>[2x]GPGSAVPFVEDWRLVQTLGEGAYGE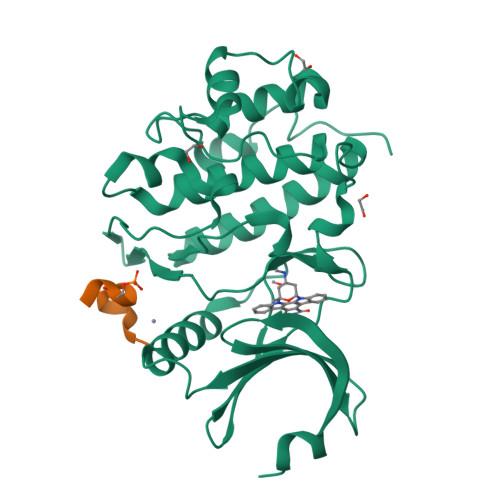VQLAVNRVTEEAVAVKIVDMKRAVDCPENIKKEICINKMLNHENVVKFYGHRREGNIQYLFLEYCSGGELFDRIEPDIGMPEPDAQRFFHQLMAGVVYLHGIGITHRDIKPENLLLDERDNLKISDFGLATVFRYNNRERLLNKMCGTLPYVAPELLKRREFHAEPVDVWSCGIVLTAMLAGELPWDQPSDSCQEYSDWKEKKTYLNPWKKIDSAPLALLHKILVENPSARITIPDIKKDRWYNKPLKKGAKRPRVTSGGVSESPSGHHHHHHHH;>MEELLNLCSGKFTSQD[2x]(3~{R})-3,4-dimethyl-3-propyl-1~{H}-1,4-benzodiazepine-2,5-dione | C14 H18 N2 O2 | 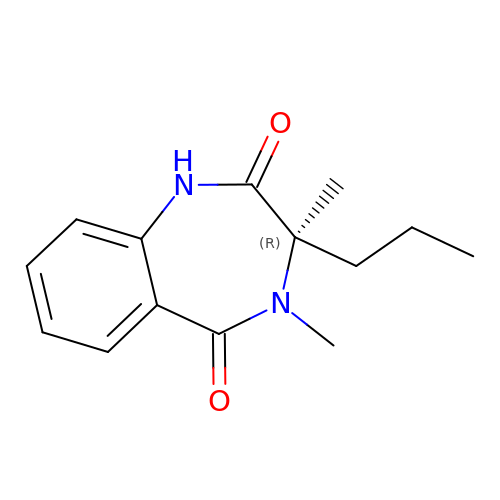CNQOZARVGPMUHF-CQSZACIVSA-N>[5x]MSEKNVSIVVAASVLSSGIGINGQLPWSISEDLKFFSKITNNKCDSNKKNALIMGRKTWDSIGRRPLKNRIIVVISSSLPQDEADPNVVVFRNLEDSIENLMNDDSIENIFVCGGESIYRDALKDNFVDRIYLTRVALEDIEFDTYFPEIPETFLPVYMSQTFCTKNISYDFMIFEKQEKKTLQNCDPARGQLKSIDDTVDLLGEIFGIRKMGNRHKFPKEEIYNTPSIRFGREHYEFQYLDLLSRVLENGAYRENRTGISTYSIFGQMMRFDMRESFPLLTTKKVFIRSIFEELIWFIKGDTNGNHLIEKKVYIWSGNGSKEYLERIGLGHREENDLGPIYGFQWRHYNGEYKTMHDDYTGVGVDQLAKLIETLKNNPKDRRHILTAWNPSALSQMALPPCHVLSQYYVTNDNCLSCNLYQRSCDLGLGSPFNIASYAI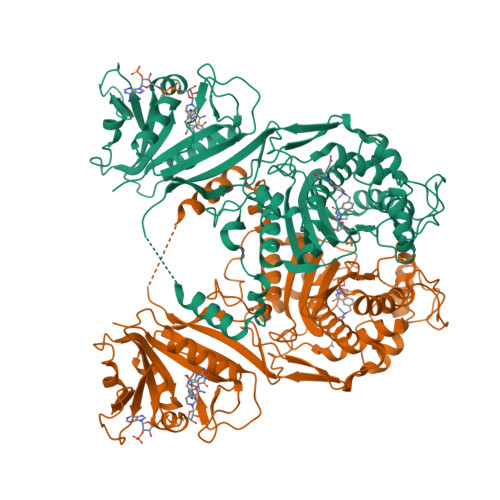LTMMLAQVCGYEPGELAIFIGDAHIYENHLTQLKEQLSRTPRPFPQLKFKRKVENIEDFKWEDIELIGYYPYPTIKMDMAV> TRLVPRG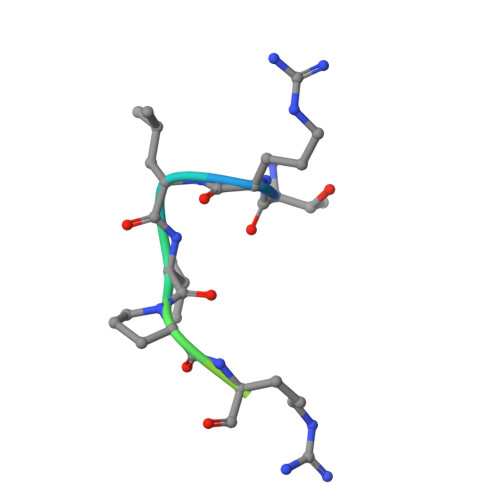SELALE>[2x]HHHHHHSSGLGVLFQGPGSKDFQGMLEYKREDEQKLVKNLILELKPRGVAVNLIPGLPAYILFM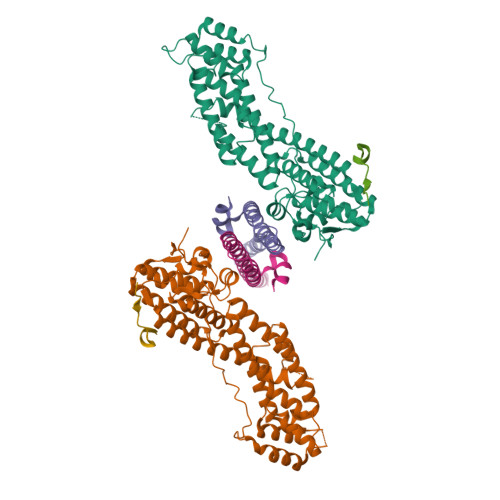CVRHADYLNDDQKVRSLLTSTINSIKKVLKKRGDDFETVSFWLSNTCRFLHCLKQYSGEEGFMKHNTSRQNEHCLTNFDLAEYRQVLSDLAIQIYQQLVRVLENILQPMIVSGMLEHETIQGVSGVKPTGLRKRTSSIADEGTYTLDSILRQLNSFHSVMSQHGMDPELIKQVVKQMFYIVGAITLNNLLLRKDMCSWSKGMQIRYNVSQLEEWLRDKNLMNSGAKETLEPLIQAAQLLQVKKKTDDDAEAICSMCNALTTAQIVKVLNLYTPVNEFEERVSVSFIRTIQMRLRDRKDSPQLLMDAKHIFPVTFPFNPSSLALETIQIPASLGLGFIARV;>[2x]GPGSEFMEDHPVREEEDGEEDEGALAKSPLQLTTDDVYDISYVVGRELMALGSDPRVTRLQFKIVRVMEMLETLVNEGSLAVEELRMERDNLKQEVEGLRKAG;>GPGSDLDTEARDQPLNSKKKKRLLSFRDVDFEEDSDHLVQPCS[2x]N-cyclopropyl-6-(furan-2-yl)-2-hydroxy-N-[(pyridin-2-yl)methyl]pyridine-3-carboxamide 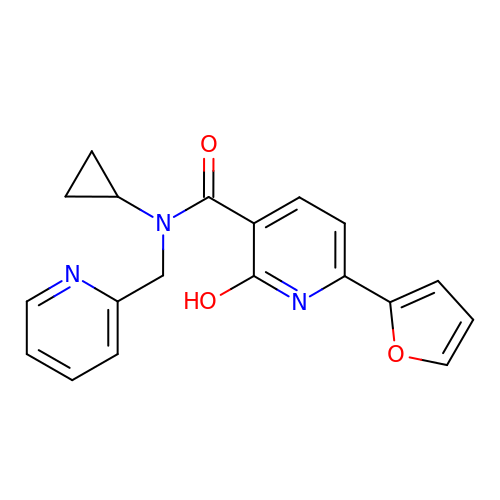| C19 H17 N3 O3 | VTYIZPVGHMMFAO-UHFFFAOYSA-N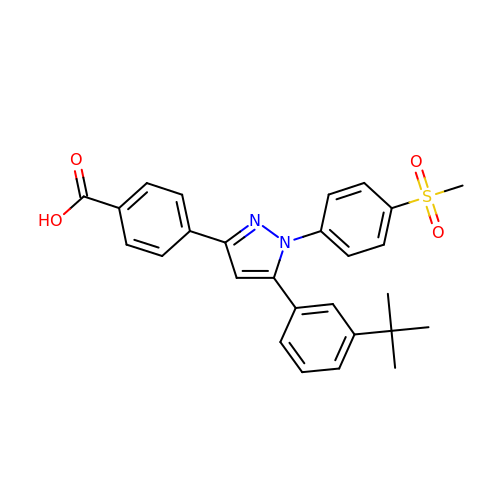4-{5-(3-tert-butylphenyl)-1-[4-(methylsulfonyl)phenyl]-1H-pyrazol-3-yl}benzoic acid | C27 H26 N2 O4 S | HPXXLUZXJROKDE-UHFFFAOYSA-N> LTGPLMLDTAPNAFDDQYEGCVNKMEEKAPLLLQEDFNMNAKLKVAWEEA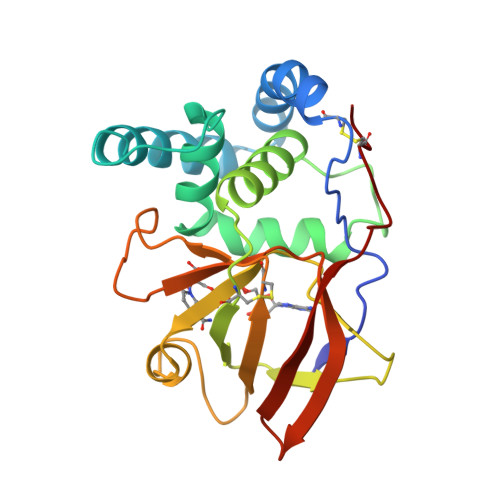KKRWNNIKPSRSYPKGFNDFHGTALVAYTGSIAVDFNRAVREFKENPGQFHYKAFHYYLTRALQLLSNGDCHSVYRGTKTRFHYTGAGSVRFGQFTSSSLSKKVAQSQEFFSDHGTLFIIKTCLGVYIKEFSFRPDQEAVLIPGYEVYQKVRTQGYNEIFLDSPKRKKSNYNCLYS> GSKDIIDVNGITIDKNAFKVTVNGAEIELTKTEYDLLYLLAENKNHVMQREQILNHVWGYNSEVETNVVDVYIRYLRNKLKPYDRDKMI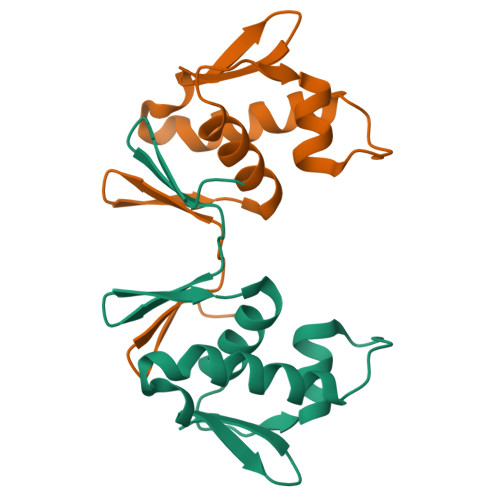ETVRGVGYVIR>SITPGTYNITNVAYTNRLIDLTGSNPAENTLIIGHHLNKTPSGYGNQQWTLVQLPHTTIYTMQ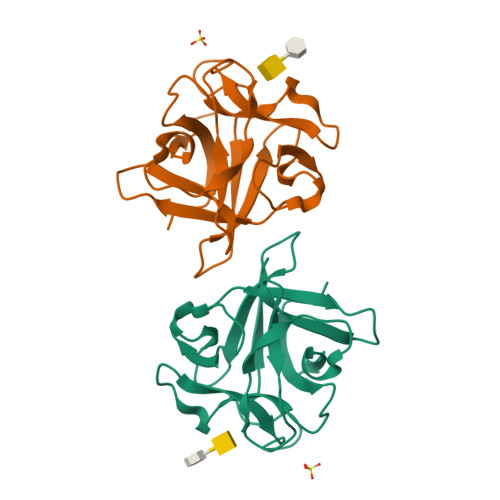AVNPQSYVRVRDDNLVDGAALVGSQQPTPVSIESAGNSGQFRIKIPNLGLALTLPSDANSTPIVLGEVDETSTNQLWAFESVSAV[2x]> NDPESALNRAVGRVADTVASGPVNTEQIPALTAVETGHTSQVVPSDTMQTRHVINYHTRSESSIENFMGRAACVYIAQYATEKVNDELDRYTNWEITTRQVAQLRRKLEMFTYMRFDLEITFVITSSQRTSTTYASDSPPLTHQVMYVPPGGPIPKSYEDFAWQTSTNPSVFWTEGNAPPRMSIPFMSVGNAYCNFYDGWSHFSQSGVYGYTTLNNMGHLYFRHVNKSTAYPVNSVARVYFKPKHVKAWVPRAPRLCPYLKARNVNFNVQGVTESRNKITLDRSTHNPLANT;> SPTVEECGYSDRVRSITLGNSTITTQECANVVVGYGVWPTYLSDHEATAVDQPTQPDVATCRFYTLESVKWESSSAGWWWKFPEALSDMGLFGQNMQYHYLGRTGYTIHVQCNASKFHQGCLLVVCVPEAEMGAATTDHAFNHTKLSNIGQAMEFSAKKSTDQTGPQTAVHNAGMGVAVGNLTIFPHQWINLRTNNSATIVMPYINSVPMDNMYRHYNFTLMVIPFAKLEHSPQASTYVPITVTVAPMCAEYNGLRLAGHQ;> GLPTMNTPGSTQFLTS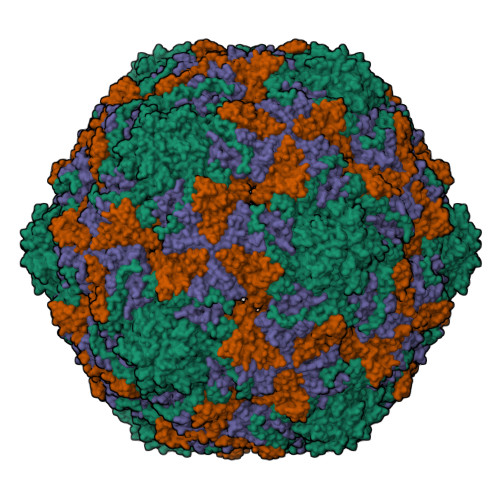DDFQSPSAMPQFDVTPEIQIPGQVRNLMEIAEVDSVVPVNNTEGHVNSMEAYRIPVRPQTSSGEQVFGFQLQPGHDSVLKHTLLGEILNYYANWSGSMKLTFMYCGAAMATGKFLIAYSPPGAGVPGSRRDAMLGTHVIWDVGLQSSCVLCVPWISQTNYRYVTSDAYTDAGYITCWYQTSIVTPPDIPTTSTILCFVSACNDFSVRLLRDTPFITQQALFQ>[4x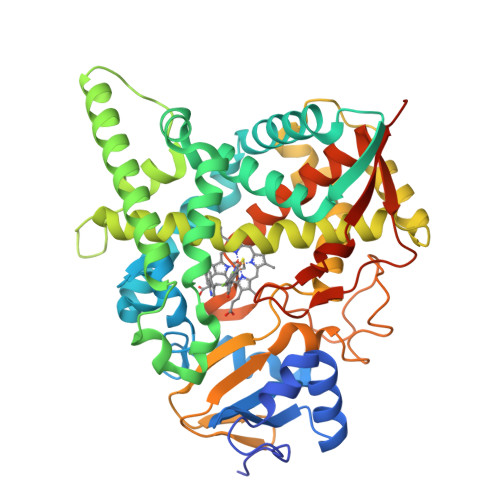]MAKKTSSKGKLPPMYPVTVPILGHIIQFGKSPLGFMQECKRQLKSGIFTINIVGKRVTIVGDPHEHSRFFLPRNEVLSPREVYSFMVPVFGEGVAYAAPYPRMREQLNFLAEELTIAKFQNFVPAIQHEVRKFMAANWDKDEGEINLLEDCSTMIINTACQCLFGEDLRKRLDARRFAQLLAKMESSLIPAAVFLPILLKLPLPQSARCHEARTELQKILSEIIIARKAAAVNKDSSTSDLLSGLLSAVYRDGTPMSLHEVCGMIVAAMFAGQHTSSITTTWSMLHLMHPANVKHLEALRKEIEEFPAQLNYNNVMDEMPFAERCARESIRRDPPLLMLMRKVMADVKVGSYVVPKGDIIACSPLLSHHDEEAFPEPRRWDPERDEKVEGAFIGFGAGVHKCIGQKFGLLQVKTILATAFRSYDFQLLRDEVPDPDYHTMVVGPTASQCRVKYIRRKAAAAHHHHHHHH> AQESLESQEQR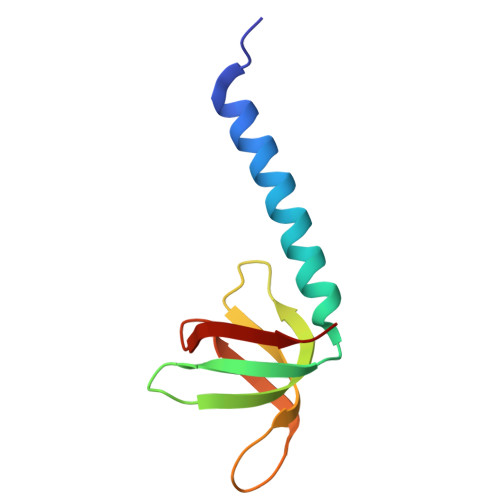ARAALRERYLRSLLAMVGHQVSFTLHEGVRVAAHFGATDLDVANFYVSQLQTPIGVQAEALLRCSDIISYTFKP>[8x]MVHLNKTIQEGDNPDLTAERLTATFDTHAMAAQIYGGEMRARRRREITAKLAEIPELHDSMPLPYMTREEKIMESARKLTVLTQRMSEIIDPTDAGELYHLNNEVLGIEGNPMALHGVMFIPALNAQASDEQQAKWLIRALRREIIGTYAQTEMGHGTNL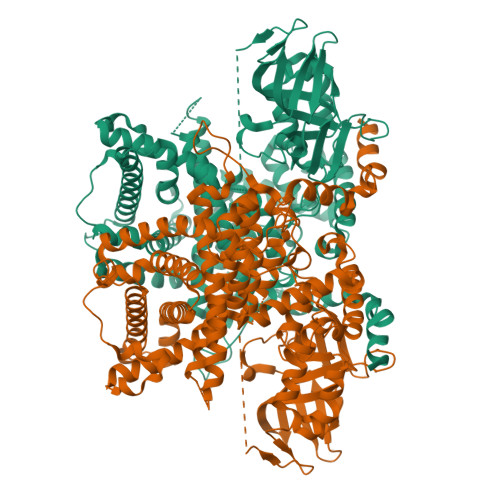QNLETTATYDIGTQEFVLHTPKITALKWWPGNLGKSSNYAVVVAHMYIKGKNFGPHTFMVPLRDEKTHKPLPGITIGDIGPKMAYNIVDNGFLGFNNYRIPRTNLLMRHTKVEADGTYIKPPHAKINYSAMVHVRSYMLTGQAIMLSYALNIATRYSAVRRQGQIDKNEPEVKVLEYQTQQHRLFPFIARAYAFQFAGAETVKLYERVLKEMKSGNVSLMADLHALTSGLKSVVTHQTGEGIEQARMACGGHGYSMASYISEIYGVAIGGCTYEGENMVMLLQLARYLVKSAALVKSGKASQLGPLVAYLGARSEPTSLIDRVPNGGITEYIKTFQHIAKRQTLKAANKFFGLMENGEKREIAWNKSSVELNRASRLHTRLFIVEAFARRVNEIGDITIKEALSDLLHLHVNYELLDVATYALEDGFMSSTQLDYVRDQLYFYLQKIRPNAVSLLDSWEFSDRELRSVLGRRDGHVYENLFKWAKESPLNKTDVLPSVDTYLKPMMEKARQSKLHHHHHHHHHH Topoisomerase II (TOP2) enzymes are essential regulators of DNA topology during DNA transcription, replication, and repair. Topoisomerase IIβ (TOP2B) plays a role in transcriptional regulation and is expressed in all cell types including post-mitotic cardiomyocytes. Both isoforms catalyze the reaction, where one DNA duplex is passed through a transient double-strand DNA break in another DNA duplex. The ATPase domain of TOP2 is highly conserved between TOP2A and TOP2B and is composed of an N-terminal strap, a β-hairpin that is unique to eukaryotic TOP2, a GHKL ATPase domain that binds and hydrolyses ATP, and a transducer domain that conveys mechanical motion to the DNA binding and cleavage core of TOP2. Here we describe the development of the obex class of TOP2 inhibitors that bind to a previously unidentified druggable pocket in the TOP2 ATPase domain to act as allosteric catalytic inhibitors by locking the ATPase domain conformation with the capability of isoform-selective inhibition.

Topoisomerase IIα (TOP2A) untangles DNA pre-catenanes during DNA replication to permit chromosome condensation and segregation in mitosis, and is primarily expressed in proliferating cells. We have been unable to obtain crystal structures of nucleotide-free eukaryotic ATPase domains, and to our knowledge none have yet been described to date. Therefore, a comparison of the AMPPNP and AMPPNP + obex inhibitor structures reveal that the obex binding site is pre-formed in the ATP-bound state of TOP2, suggesting that topobexin (9) fits into TOP2B like a key into a lock and blocks subsequent conformational changes that could otherwise occur upon ATP hydrolysis. Residues surrounding the 5c pocket are largely unchanged from those observed in its absence, suggesting the ATP-bound state can easily accommodate 5c. Interestingly, 5c induces a slight shift in Y72 of TOP2A compared to apo TOP2A due to packing of this non-conserved residue against the hydroxyethyl group, while the equivalent C88 residue in TOP2B is located 4.7 Å away and does not interact with 5c.

>[2x]SNASVERIYQKKTQLEHILLRPDTYIGSVELVTQQMWVYDEDVGINYREVTFVPGLYKIFDEILVNAADNKQRDPKMSCIRVTIDPENNLISIWNNGKGIPVVEHKVEKMYVPALIFGQLLTSSNYDDDEKKVTGGRNGYGAKLCNIFSTKFTVETASREYKKMFKQTWMDNMGRAGEMELKPFNGEDYTCITFQPDLSKFKMQSLDKDIVALMVRRAYDIAGSTKDVKVFLNGNKLPVKGFRSYVDMYLKDKLDETGNSLKVIHEQVNHRWEVCLTMSEKGFQQISFVNSIATSKGGRHVDYVADQIVTKLVDVVKKKNKGGVAVKAHQVKNHMWIFVNALIENPTFDSQTKENMTLQPKSFGSTCQLSEKFIKAAIGCGIVESILNWVKFKAQVQLN>HHHHHHHMIVLFVDFDYFYAQVEEVLNPSLKGKPVVVCVFSGRFEDSGAVATANYEARKFGVKAGIPIVEAKKILPNAVYLPMRKEVYQQVSSRIMNLLREYSEKIEIASIDEAYLDISDKVRDYREAYNLGLEIKNKILEKEKITVTVGISKNKVFAKIAADMAKPNGIKVIDDEEVKRLIRELDIADVPGIGNITAEKLKKLGINKLVDTLSIEFDKLKGMIGEAKAKYLISLARDEYNEPIRTRVRKSIGRIVTMKRNSRNLEEIKPYLFRAIEESYYKLDKRIPKAIHVVAVTEDLDIVSRGRTFPHGISKETAYSESVKLLQKILEEDERKIRRIGVRFSKFIEAIGLDK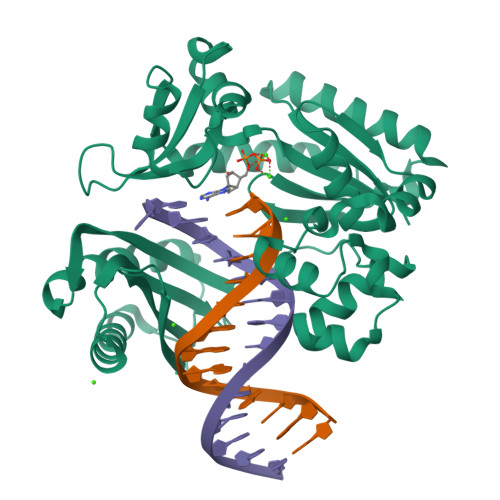FFDT[2x]> GAGCAXG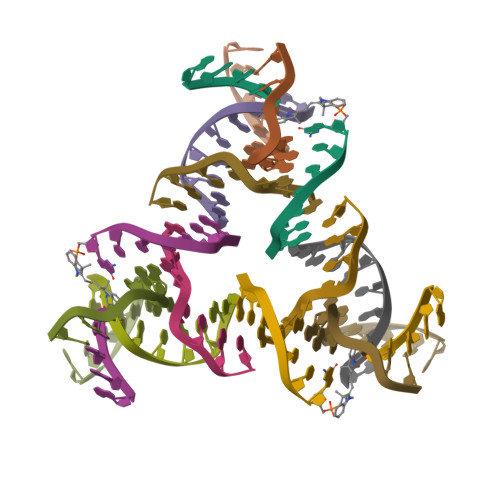CCTGTA;> ACACCGT;> TCTGATGTGGCTGC;> CGGACATCA The S. cerevisiae plasma membrane H+-ATPase, Pma1, is a P3A-type ATPase and the primary protein component of the membrane compartment of Pma1 (MCP). Like other plasma membrane H+-ATPases, Pma1 assembles and functions as a hexamer, a property unique to this subfamily among the larger family of P-type ATPases. Like all other P-type ATPases, the plasma membrane H+-ATPase has a transmembrane domain (TMD) composed of ten transmembrane α-helices (TMs), an actuator domain (A-domain), a nucleotide-binding domain (N-domain), and a phosphorylation domain (P-domain). Remarkably, we found that the Pma1 hexamer encircles a liquid-crystalline membrane domain composed of 57 ordered lipid molecules.

We determined the cryo-EM structure of autoinhibited Pma1 hexamer at pH 7.4 to 3.2 Å resolution without imposing any symmetry; we term this structure Pma1-pH7-C1. We found that the TMD and P-domains are well ordered and symmetric, while the A-and N-domains are asymmetric and flexible. At pH 7.4, the carboxyl-terminal regulatory α-helix binds to the phosphorylation domains of two neighboring Pma1 subunits, locking the hexamer in the autoinhibited state. The C-terminal peptide (880–918, termed C-tail) forms two α-helices in the autoinhibited structure of Pma1. The first C-tail helix is short, horizontal, and partially embedded in the membrane. The second C-tail helix is longer and mediates the interaction between the P-domain and the P-domain of the neighboring subunit. In the autoinhibited state, S911, H914, and E917 of helix-i interact with K566, N577, Y579, and R583 of the P-domain to the left, and R898, E901, and D902 of helix-i interact with S595', D599', and R625' of the neighboring P-domain to the right. Major interactions include two inter-molecular salt bridges (R898:D599' and E901:R625') and an intramolecular hydrogen bond (S911:K566). We have shown that autoinhibition of Pma1 is achieved primarily by the C-tail helix-i simultaneously binding and constraining the movement of two neighboring P-domains. In the autoinhibited state, D730 is surrounded by R695, N154, and Q125 but these residues are outside the range of direct interaction.

>MTDTSSSSSSSSASSVSAHQPTQEKPAKTYDDAASESSDDDDIDALIEELQSNHGVDDEDSDNDGPVAAGEARPVPEEYLQTDPSYGLTSDEVLKRRKKYGLNQMADEKESLVVKFVMFFVGPIQFVMEAAAILAAGLSDWVDFGVICGLLMLNAGVGFVQEFQAGSIVDELKKTLANTAVVIRDGQLVEIPANEVVPGDILQLEDGTVIPTDGRIVTEDCFLQIDQSAITGESLAVDKHYGDQTFSSSTVKRGEGFMVVTATGDNTFVGRAAALVNKAAGGQGHFTEVLNGIGIILLVLVIATLLLVWTACFYRTNGIVRILRYTLGITIIGVPVGLPAVVTTTMAVGAAYLAKKQAIVQKLSAIESLAGVEILCSDKTGTLTKNKLSLHEPYTVEGVSPDDLMLTACLAASRKKKGLDAIDKAFLKSLKQYPKAKDALTKYKVLEFHPFDPVSKKVTAVVESPEGERIVCVKGAPLFVLKTVEEDHPIPEDVHENYENKVAELASRGFRALGVARKRGEGHWEILGVMPCMDPPRDDTAQTVSEARHLGLRVKMLTGDAVGIAKETCRQLGLGTNIYNAERLGLGGGGDMPGSELADFVENADGFAEVFPQHKYRVVEILQNRGYLVAMTGDGVNDAPSLKKADTGIAVEGATDAARSAADIVFLAPGLSAIIDALKTSRQIFHRMYSYVVYRIALSLHLEIFLGLWIAILDNSLDIDLIVFIAIFADVATLAIAYDNAPYSPKPVKWNLPRLWGMSIILGIVLAIGSWITLTTMFLPKGGIIQNFGAMNGIMFLQISLTENWLIFITRAAGPFWSSIPSWQLAGAVFAVDIIATMFTLFGWWSENWTDIVTVVRVWIWSIGIFCVLGGFYYEMSTSEAFDRLMNGKPMKEKKSTRSVEDFMAAMQRVSTQHEKET[6x]>SNVEPVGRLHIFSGAHGPEKDFPLHLGKNVVGRMPDCSVALPFPSISKQHAEIEILAWDKAPILRDCG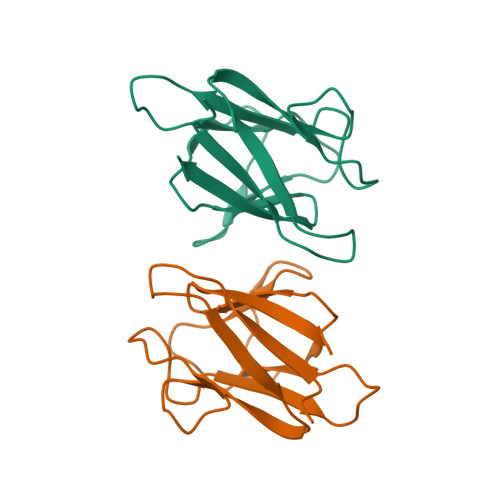SLNGTQILRPPKVLSPGVSHRLRDQELILFADLLCQYHRLDVSLP[2x]>MAYSQGGGKKKVCYYYDGDIGNYYYGQGHPMKPHRIRMTHNLLLNYGLYRKMEIYRPHKATAEEMTKYHSDEYIKFLRSIRPDNMSEYSKQMQRFNVGEDCPVFDGLFEFCQLSTGGSVAGAVKLNRQQTDMAVNWAGGLHHAKKSEASGFCYVNDIVLAILELLKYHQRVLYIDIDIHHGDGVEEAFYTTDRVMTVSFHKYGEYFPGTGDLRDIGAGKGKYYAVNFPMRDGIDDESYGQIFKPIISKVMEMYQPSAVVLQCGADSLSGDRLGCFNLTVKGHAKCVEVVKTFNLPLLMLGGGGYTIRNVARCWTYETAVALDCEIPNELPYNDYFEYFGPDFKLHISPSNMTN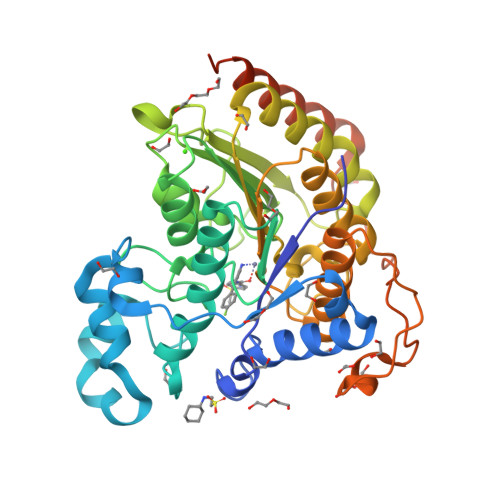QNTPEYMEKIKQRLFENLRMLPHAPGVQMQAIPEDAVHEDSGDEDGEDPDK[3x]>[2x]MKHHHHHHHMVSTLKPLKIGKHTIKFPIFQGGMGVGISWDELAGNVAKEGALGVISAVGTGYYKNMRFVERIVAKKPFEALNFYSKKALNEIFANARKICGNNPLGANILYAINDYGRVLRDSCEAGANIII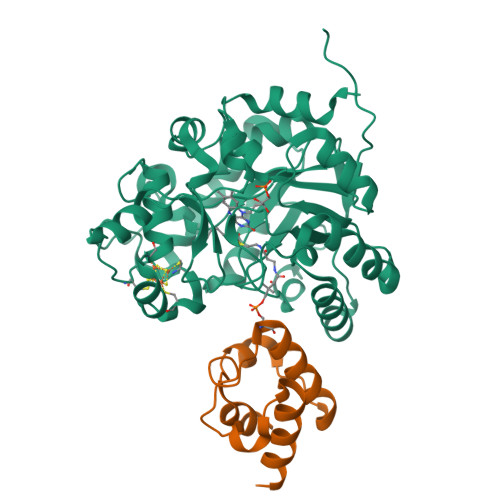TGAGLPTNMPEFAKDFSDVALIPIISSAKALKILCKRWSDRYKRIPDAFIVEGPLSGGHQGFKYEDCFKEEFRLENLVPKVVEASKEWGNIPIIAAGGIWDRKDIDTMLSLGASGVQMATRFLGTKECDAKVYADLLPTLKKEDILLIKSPVGYPARAINTGVIKRIEEGNAPKIACVSNCVAPCNRGEEAKKVGYCIADGLGRSYLGNREEGLYFTGANGYRVDKIISVHELIKELTEG;>GTSSMGYLMALFEDIQAVIAEQLNVDAAQVTPEAEFVKDLGADSLDVVELIMALEEKFGIEIPDEQAEKIVNVGDVVKYIEDNKLA[2x]N-(8-methyl-2-phenylimidazo[1,2-a]pyridin-3-yl)-2-(3-oxo-2,3-dihydro-4H-1,4-benzothiazin-4-yl)acetamide | C24 H20 N4 O2 S | 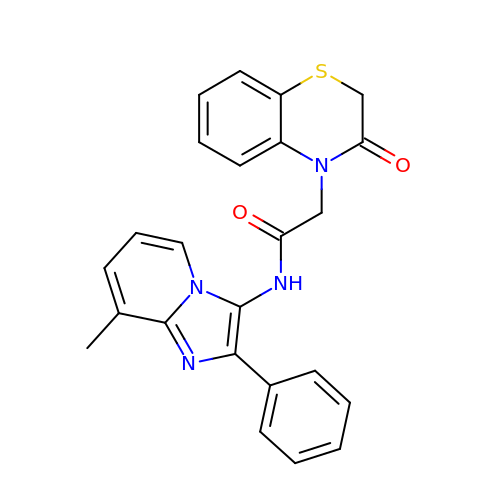MSTWIUSEUCGNEI-UHFFFAOYSA-N> MTSKTKNIDDIPPEIKEEMIQLYHDLPGIENEYKLIDKIGEGTFSSVYKAKDITGKITKKFASHFWNYGSNYVALKKIYVTSSPQRIYNELNLLYIMTGSSRVAPLCDAKRVRDQVIAVLPYYPHE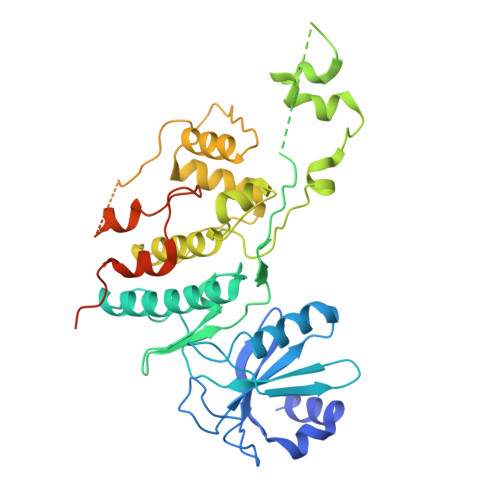EFRTFYRDLPIKGIKKYIWELLRALKFVHSKGIIHRDIKPTNFLFNLELGRGVLVDFGLAEAQMDYKSMISSQNDYDNYANTNHDGGYSMRNHEQFCPCIMRNQYSPNSHNQTPPMVTIQNGKVVHLNNVNGVDLTKGYPKNETRRIKRANRAGTRGFRAPEVLMKCGAQSTKIDIWSVGVILLSLLGRRFPMFQSLDDADSLLELCTIFGWKELRKCAALHGLGFEASGLIWDKPNGYSNGLKEFVYDLLNKECTIGTFPEYSVAFETFGFLQQELHDRMSIEPQLPDPKTNMDAVDAYELKKYQEEIWSDHYWCFQVLEQCFEMDPQKRSSAEDLLKTPFFNELNENTYLLDGESTDEDDVVSSSEADLLDKDVLLISE>[4x]MGHHHHHHGGTILVVTGTGTGVGKTVVCAALASA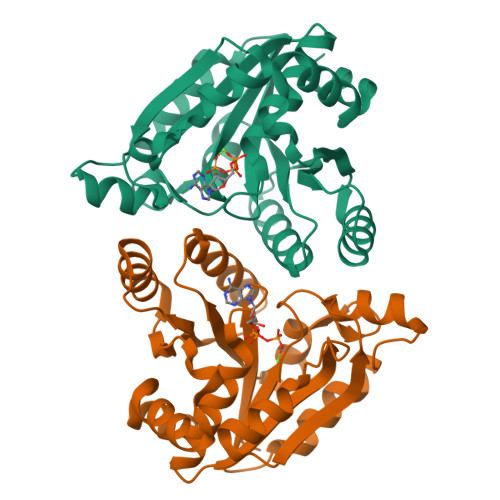ARQAGIDVAVCKPVQTGTARGDDDLAEVGRLAGVTQLAGLARYPQPMAPAAAAEHAGMALPARDQIVRLIADLDRPGRLTLVEGAGGLLVELAEPGVTLRDVAVDVAAAALVVVTADLGTLNHTKLTLEALAAQQVSCAGLVIGSWPDPPGLVAASNRSALARIAMVRAALPAGAASLDAGDFAAMSAAAFDRNWVAGLVG C. elegans SAS-6 physically interacts with SAS-5, a protein that shuttles rapidly between the cytoplasm and centrioles throughout the cell cycle. The presence of SAS-6 and SAS-5 at centrioles is essential for formation of the central tube, a cylindrical structure at the core of the emerging centriole. Overall, these findings led us to conclude that the segment between residues 125–265 contains two independently folded domains and encompasses all structured elements of SAS-5.

The SAS-5 Implico domain comprises a novel type of protein dimer. Each chain features three α-helices (A1 to A3 and B1 to B3) that interact in a pairwise manner (A1–B3, A2–B2 and A3–B1). Proline residues at the linkers between helices allow for tight 90° turns, resulting in a very compact dimer of just ∼4 nm in diameter. We found that this newly recognized domain is highly conserved amongst Caenorhabditis species. Structural and biophysical analysis suggests that SAS-5 can form tight dimers through its Implico domain, a novel dimerization interface with no known homologs outside SAS-5 proteins. These dimers cannot be disrupted even when diluting the protein to concentrations as low as 20 nM. We envision that SAS-5 would readily dimerize even at low concentrations via the Implico domain, as oligomerization of this domain is tighter compared to that of the SAS-5 coiled coil. As anticipated, coiled coil disruptions in either SAS-52–265 L141E or L141E/M167E mutants yielded a stable dimer in SEC-MALS experiments, mediated by the Implico domain. Furthermore, we found that a SAS-52–265 I247E mutant, where the Implico domain is disrupted, displayed a single-step thermal unfolding profile as measured by CD with a Tm similar to that of the SAS-5 coiled coil in isolation (compare Figure 5A). SEC-MALS analysis of the same construct shows a concentration-dependent trimerization, again consistent with formation of just the SAS-5 coiled coil. Our work shows that formation of these tight SAS-5 dimers through the Implico domain is necessary for SAS-5 localization to centrioles.

>[2x]GPLGSKIASAREVIKRDGVIPPEALTIIEQRLRSDPMFRQQIDNVLADAECDANRAAYSP>[4x]GSHMESFLLSKVSFVIKKIRLEKGMTQEDLAYKSNLDRTYISGIERNSRNLTIKSLE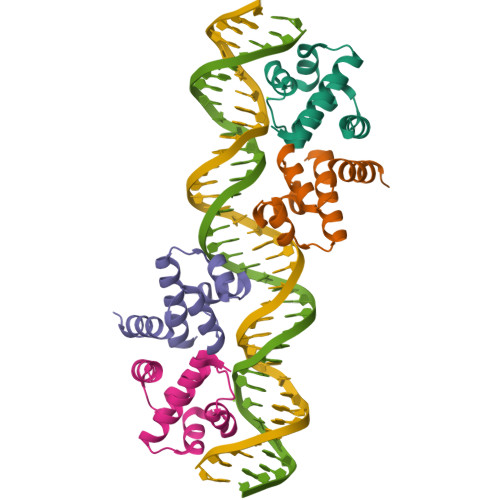LIMKGLEVSDVVFFEMLIKEILKHD The target protein used in this study is the computationally stabilized haloalkane dehalogenase DhaA115 designed previously using the web server FireProt. Eleven mutations that were originally introduced in the wild type increased its apparent melting temperature (Tmapp) to approx. 73 °C (ΔTmapp ∼ 23 °C), making it the most stable haloalkane dehalogenase to date. First, DhaA115 displays activity toward a broad range of halogenated substrates, many of which are toxic and carcinogenic compounds persistent in the environment, e.g., 1,2-dichloroethane and 1,2-dibromoethane. This makes the enzyme particularly valuable for biotechnological applications that detoxify and degrade harmful pollutants.

Following the experimental validation of all FireProt designs, we removed the destabilizing mutations L161M, I163L from DhaA216 and obtained the most stable FireProt variant, DhaA223, with 6 °C higher Tmapp compared to DhaA115. We obtained diffraction-quality crystals of DhaA223 and DhaA231 enzymes that belonged to the space groups P1211 and P212121 and diffracted at 1.5 and 1.3 Å resolution, respectively. The positioning of catalytic pentad residues was not disturbed, which is a prerequisite for efficient catalysis. Here, we show that the protein backbones of DhaA223 and DhaA231 superpose well with that of the DhaA115, although some minor changes are observed in the hinge regions between the helical cap domain and the hydrolase core. The crystal structures of DhaA223 and DhaA231 thus suggest that stabilization was achieved via strengthening intricate networks of residue-to-residue interactions, stabilizing the αβα-sandwich architecture. A notable example includes residues 184 and 197, where mutation of hydrophobic valines to glutamic acids created local hydrogen-bond networks involving water molecules. Specifically, this translates to approx. 7-, 12-, and 5-times longer half-lives at 70 °C of DhaA222, 223, and 231, respectively, compared to the 8-minute half-life of DhaA115 at this temperature. Consequently, DhaA222 and DhaA223 reach similar levels of catalytic efficiency at 60 °C when adjusted for the substrate inhibition (i.e., kcat·Ksi/Km), which is 3–4 times higher compared to DhaA115 and DhaA231. The substrate inhibition of DhaA222 and DhaA231 is exergonic at the whole temperature range, in contrast to DhaA223, for which it becomes energetically unfavorable at high temperatures.

>[6x]MSEIGTGFPFDPHYVEVLGSRMHYVDVGPRDGTPVLFLHGNPTSSYLWRNIIPHVAPSHRCIAPDLIGMGKSDKPDLDYRFDDHVRYLDAFIEALGLEEVVLVIHDWGSALGFHWAKRNPERVKGIAFMEFIRPIPTWDEWPEFARELFQAFRTPDVGRELIIDYNAFIEIILPKFVVRPLTEEEMDHYREPFLKPEWREPLWRFPNELPINGEPADIWALVEAYMNWLHQSPVPKLLFWGTPGVLIPPAEAARLAESLPNLKTVFIGPGLHYLQEDNPDLIGSEIARWLPALHHHHHH>[2x]SGGNPGERLRKKKWDLSELPKFEKNFYVEHPEVARLTPYEVDELRRKKEITVRGGDVCPKPVFAFHHANFPQYVMDVLMDQHFTEPTPIQCQGFPLALSGRDMVGIAQTGSGKTLAYLLPAIVHINHQPYLERGDGPICLVLAPTRELAQQVQQVADDYGKCSRLKSTCIYGGAPKGPQIRDLERGVEICIATPGRLIDFLESGKTNL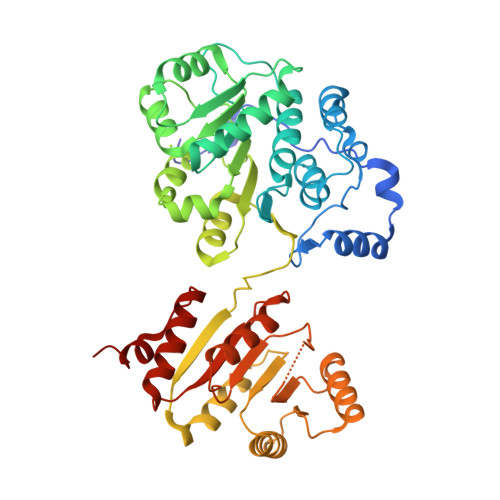RRCTYLVLDEADRMLDMGFEPQIRKIVDQIRPDRQTLMWSATWPKEVRQLAEDFLRDYTQINVGNLELSANHNILQIVDVCMESEKDHKLIQLMEEIMAEKENKTIIFVETKRRCDDLTRRMRRDGWPAMCIHGDKSQPERDWVLNEFRSGKAPILIATDVASRGLDVEDVKFVINYDYPNSSEDYVHRIGRTARSTNKGTAYTFFTPGNLKQARELIKVLEEANQAINPKLMQLVDHRG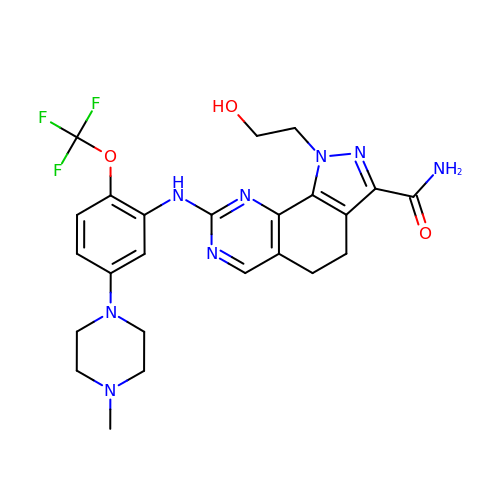1-(2-HYDROXYETHYL)-8-[[5-(4-METHYLPIPERAZIN-1-YL)-2-(TRIFLUOROMETHOXY)PHENYL]AMINO]-4,5-DIHYDROPYRIMIDO[5,4-G]INDAZOLE-3-CARBOXAMIDE | C24 H27 F3 N8 O3 | QHLVBNKYJGBCQJ-UHFFFAOYSA-N>[2x]GPNCAPGKVKLFRASEPILSVLMWGVNHTINELSNVPVPVMLMPDDFKAYSKIKVDNHLFNKENLPSRFKFKEYCPMVFRNLRERFGIDDQDYQNSVTRSAPINSDSQGRCGTRFLTT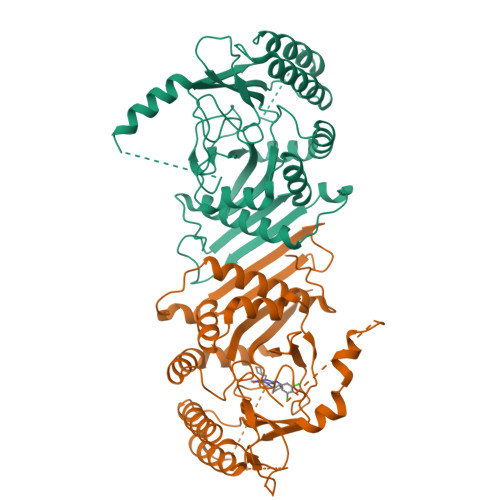YDRRFVIKTVSSEDVAEMHNILKKYHQFIVECHGNTLLPQFLGMYRLTVDGVETYMVVTRNVFSHRLTVHRKYDLKGSTVAREASDKEKAKDLPTFKDNDFLNEGQKLHVGEESKKNFLEKLKRDVEFLAQLKIMDYSLLVGIHDVDRAEQEEMEVEERAEDEECENDGVGGNLLCSYGTPPDSPGNLLSFPRFFGPGEFDPSVDVYAMKSHESSPKKEVYFMAIIDILTPYDTKKKAAHAAKTVKHGAGAEISTVNPEQYSKRFNEFMSNILT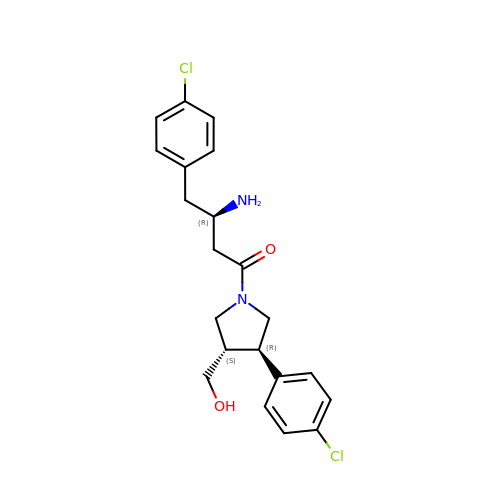(3R)-3-amino-4-(4-chlorophenyl)-1-[(3R,4S)-3-(4-chlorophenyl)-4-(hydroxymethyl)pyrrolidin-1-yl]butan-1-one | C21 H24 Cl2 N2 O2 | ZFSKJGRASNTEBX-DBVUQKKJSA-N> GHPYYLRSFLVVLKTVLENEDDMLLFDEQEKGIVTKFYQLSATGQKLYVRLFQRKLSWIKMTKLEYEEIALDLTPVIEELTNAGFLQTESELQELSEVLELLSAPELKSLAKTFHLVNPNGQKQQLVDAFLKLAKQRSVCTWGKNKPGIGAVILKRAKALAGQSVRICKGPRAVFSRILLLFSLTDSMEDEDAACGGQGQLSTVLLVNLGRMEFPSYTINRKTHIFQDRDDLIRYAAATHMLSDISSAMANGNWEEAKELAQCAKRDWNRLKNHPSLRCHEDLPLFLRCFTVGWIYTRILSRFVEILQRLHMYEEAVRELESLLSQRIYCPDSRGRWWDRLALNLHQHLKRLEPTIKCITEGLADPEVRTGHRLSLYQRAVRLRESPSCKKFKHLFQQLPEMAVQDVKHVTITGRLCPQRGMCKSVFVMEAGEAADPTTVLCSVEELALAHYRRSGFDQGIHGEGSTFSTLYGLLLWDIIFMDGIPDVFRNACQAFPLDLCTDSFFTSRRPALEARLQLIHDAPEESLRAWVAATWHEQEGRVASLVSWDRFTSLQQAQDLVSCLGGPVLSGVCRHLAADFRHCRGGLPDLVVWNSQSRHFKLVEVKGPNDRLSHKQMIWLAELQKLGAEVEVCHVVAVGGSENLYFQ

In 2010, four groups identified a novel FA-associated nuclease, FAN1, that directly binds to monoubiquitinated FANCD2, participating in ICL repair. FAN1 is a structure-specific nuclease and possesses preferential endonuclease activity toward 5′ flap structures and a weaker 5′-3′ exonuclease activity in vitro and has been hypothesized to cleave DNA in multiple steps. The FAN1 nuclease is recruited to the damage foci through its UBZ domain and acts as an effector by executing one or more DNA strand incisions during ICL repair. Previous studies have indicated that the depletion of FAN1 or mutations that defect the nuclease activity cause hypersensitivity to ICL-inducing agents and defects in HR, suggesting its significance for efficient ICL repair.

Here, we report the crystal structure of human FAN1 lacking the highly flexible UBZ domain (referred to hereafter as hFAN1 for brevity). The crystal structure of hFAN1 was determined at 2.8 Å resolution using the single-wavelength anomalous diffraction (SAD) method. The asymmetric unit contains one molecule encompassing residues 371–1010 with four disordered loops (residues 506–516, 557–569, 755–765 and 792–809). The overall structure of hFAN1 consists of an SAP-containing N-terminal domain (NTD, residues 371–594), a middle tetratricopeptide repeat domain (TPR domain, residues 595–772) and a C-terminal viral replication and repair nuclease domain (VRR_nuc domain, residues 773–1010) and folds into the shape of a short handled scoop. In the active site of PaFAN1, residues D507, E522 and K524 of the typical PDXn(D/E)XK motif, together with a nearby residue, E386, coordinate the dimetal group, and these four residues are strictly conserved in hFAN1 (D960, E975, K977 and E834). In addition, the nearly identical orientation of these residues suggests that they may share a common DNA cleavage mechanism. In addition, the notably disordered loop between α11 and α12 is close to the equivalent position of the “wedge” that protrudes into the substrate junction in the PaFAN1 structure, suggesting that this loop in hFAN1 may be involved in DNA-induced conformational changes. In contrast, at the equivalent position in hFAN1, the hole is much smaller and unlikely to allow ssDNA passage. Thus, our structure supports the notion that hFAN1 is unlikely to sequester 5′ flap DNA via a threading mechanism.Narazaciclib | C24 H27 N7 O 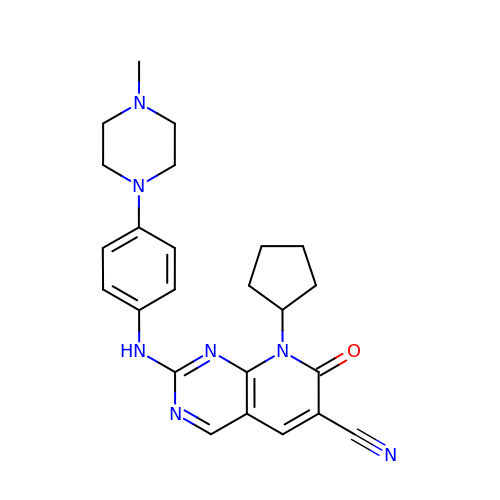| VADOZMZXXRBXNY-UHFFFAOYSA-N> SIQGTSLLTQSPASLSTYNDQSVSFVLENGSYVINVDDSGKDQEQDQVLLRYYESPSPASQSGDGVDGKKLMVNMSPIKDTDIWLHANDKDYSVELQRGDVSPPEQAFFVLHKKSSDFV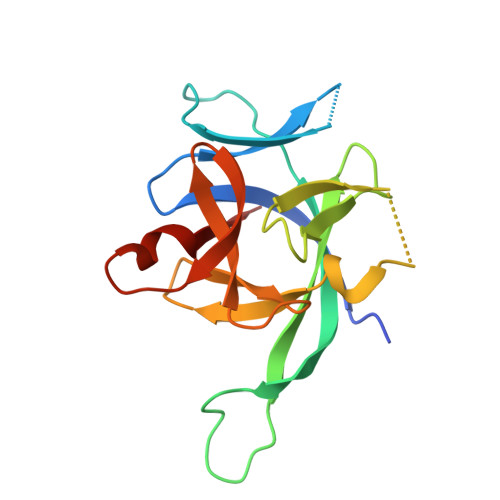SFESKNLPGTYIGVKDNQLALVEEKDESSNNIMFKLSKI>[2x]MSTVRRLEGKVALITGGAGNIGEVITRRFLAEGATVVITGRNAEKLAVYRRRLIDEERVAPERVVALRMDGSDIAQVRAGVAQIVHGGTDVPIPLHRIDILVNNAGSAGPRRRLVDIPLEPSEVQPPDSETLAQAVGNLVGITWNLTRAAAPHMPSGSSVINISTIFSRTDYYGRIAYVAPKAALNALSDGLARE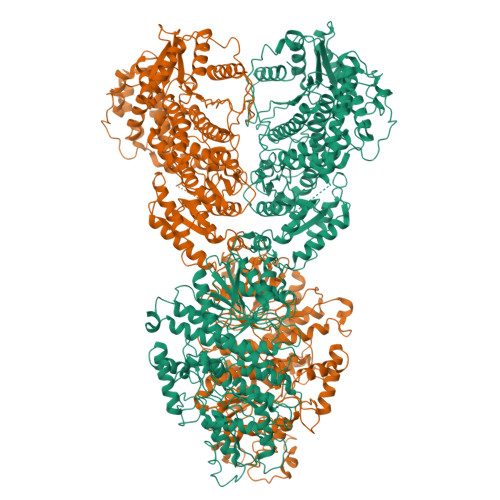LGVRGIRVNTIYPGPIESERIYTMFQAMDALKGQPEGDTASGFLRMMRLSRIDQNGEVVKRFPSPVDVANTAVLLASDESAAFTGHAFEVTHGMEVPTESRTTFVSRPGLRSVDATGKVILICAGDQVDDAVALADTLRSCRATVVIGFRDPRALEKASVLLREPRHALAADMYGRPTMTAEARLVRLDPLDPRAAAQTLEQIHAELGAIHHAVVLPGQSRHAPSASLIEVDDQVVERFLHQELVGTIALARELARFWEEYPSGSSMHRVLFVSNPDDQQGNQYSHILRAAVEQLVRVWRHESEYDSVNPAHQQEGQSSAAVWANQLIRYVNNEMANLDFTCAWVAKLLGSDRRIAEINLYLPEEIVGTIGVHNPGFGWAESLFGLHMGKVALITGGSAGIGGQIGRLLALSGAHVMLAARNADQLEQMRASIVREVRDASYPDAESRVAIFPGSDVSDIDGLERLVNHTVRVFGKVDYLINNAGIAGAEEMVIDMPVDAWRHTLRANLISNYALLRRLAPQMKAAGGAYVLNVSSYFGGEKYVAIPYPNRSDYAVSKAGQRAMVESLARFLGPEIQINAIAPGPVEGERLKGAGSRPGLFMRRARLILENKRLNEVFAALLAARHEGATIADLLPDLFANDIQSIANSAAMPAPLRRLATMLRETSDAGGSAQSYLMNATIARKLLNRLENGGYITLHDRRALTVEPPEPFFTEAQIEREAIKVRDGILGMLHLQRMPTEFDVALATVFYLADRNVTGETFHPSGGLRFERTVTEGELFGKPGQQRLERLKGSVVYLIGEHLRQHLVLLARTFLDEIHVARVVLLTETTQAATDLAAELSDYEAAGRFVVIPTCGDIEGGIDRAMAEYGRPGPVISTPFRPLPDRALSARNGDWSSVLTTAEFEELVEQQITHHFRVARKAGLIEGANVTLVTPPTSARSTSEEFALANFVKTTLHALTATAGAESERTVPHVPVNQVDLTRRARSEEPRTPSEEEEELQRFVNAVLLTSAPLPTPLESRYRARIYRGNAITV>[2x]MTISRRDFLNGVALTIAAGLTPAEILRAAPGGRYYPPALTGLRGSHPGAFEVAHQMGWEKKTFDVDHLPIEEEYDLVVVGGGISGLAAAWFYRERHPAARILVIENHDDFGGHAKRNEFQAGGRTILGYGGSESLQSPNALYSEDAKHLLKRLGVELKRFETAFDTDFYPGLGLSRAVFFDKASFGVDKLVSGDPTPMVADEVPRDRLNARSWRAFIGDFPLSREDREALIALYESPRDYLAGKSVEEKETYLAKTSYRDYLLKNVGLSETSVKYFQGRSNDFSALGADALPAADAYAAGFPGFDALGLPQPSEEAQAEMDEPYIYHFPDGNAS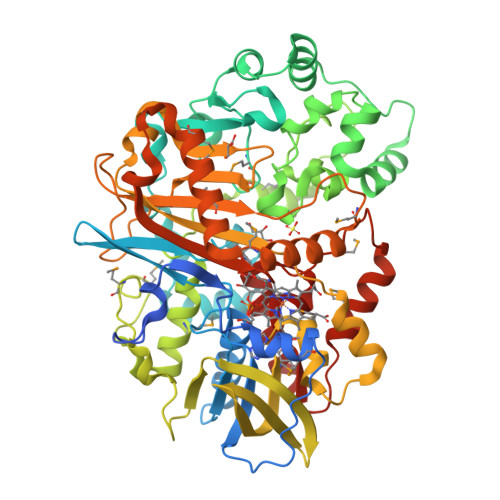LARLMVRDLIPAVAPGRGMEDIVMARFDYSKLDLAGHPVRLRLNSTAVSVRNRAGGVDVGYSRAGRLHRVRGKHCVMACYNMMVPYLLRDLSEEQAHALSQNVKFPLVYTKVLLRNWQAWKTLGIHEIYAPTLPYSRIKLDFPVDLGSYRHPRDPRQPIGVHMVYVPTTPNAGMDARTQARVGRSKLYAMSFEQLEKDIRDQLQAMLGPAGFDHRRDITGITVNRWSHGYSYFMNTLYDDEAESEALMELARSKVGNVAIANSDAAWDAYAHAAIDQAVRAVRELG> MAWPKVQPEVNIGVVGHVDHGKTTLVQAITGIWTSKHSEELKRGMTIKLGYAETNIGVCESCK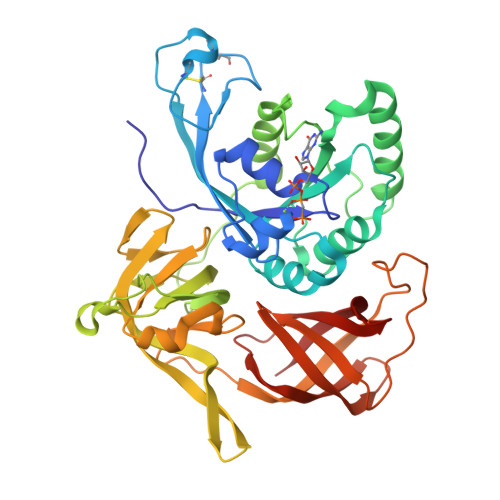KPEAYVTEPSCKSCGSDDEPKFLRRISFIDAPGHEVLMATMLSGAALMDGAILVVAANEPFPQPQTREHFVALGIIGVKNLIIVQNKVDVVSKEEALSQYRQIKQFTKGTWAENVPIKPVSALHKINIDSLIEGIEEYIKTPYRDLSQKPVMLVIRSFDVNKPGTQFNELKGGVIGGSIIQGLFKVDQEIKVLPGLRVEKQGKVSYEPIFTKISSIRFGDEEFKEAKPGGLVAIGTYLDPSLTKADNLLGSIITLADAEVPVLWNIRIKYNLLERVVGAKEMLKVDPIRAKETLMLSVGSSTTLGIVTSVKKDEIEVELRRPVAVWSNNIRTVISRQIAGRWRMIGWGLVEI>[2x]AEVPLPQLRAYTVDASWLQPMAPLQIADHTWQIGTEDLTALLVQTPDGAVLLDGGMPQMASHLLDNMKARGVTPRDLRLILLSHAHADHAGPVAELKRRTGAKVAANAESAVLLARGGSDDLHFGDGITYPPANADRIVMDGEVITVGGIVFTAHFMAGHTPGSTAWTWTDTRNGKPVRIAYADSLSAPG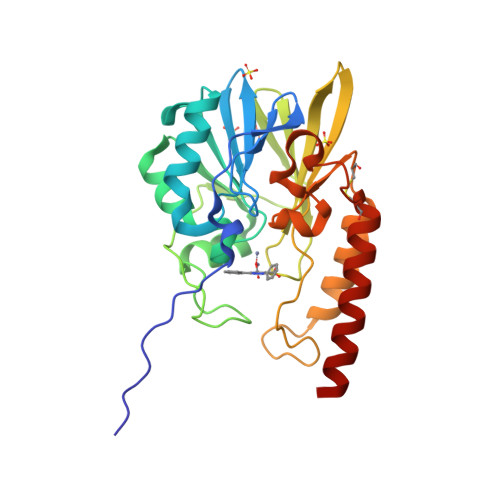YQLQGNPRYPHLIEDYRRSFATVRALPCDVLLTPHPGASNWDYAAGARAGAKALTCKAYADAAEQKFDGQLAKETAGAR>[2x]AVTPPPEKFNFAEHLLQTNRVRPDKTAFVDDISSLSFAQLEAQTRQLAAALRAIGVKREERVLLLMLDGTDWPVAFLGAIYAGIVPVAVNTLLTADDYAYMLEHSRAQAVLVSGALHPVLKAALT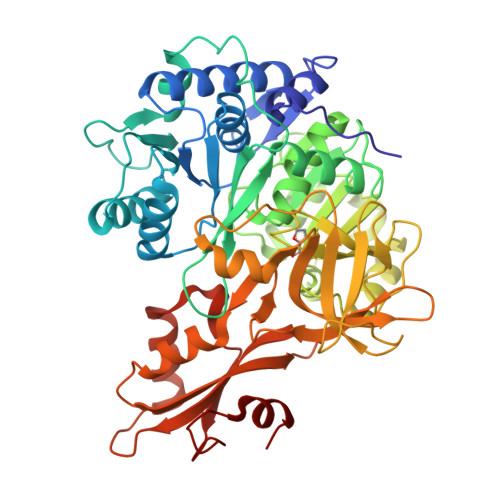KSDHEVQRVIVSRPAAPLEPGEVDFAEFVGAHAPLEKPAATQADDPAFWLYSSGSTGRPKGVVHTHANPYWTSELYGRNTLHLREDDVCFSAAKLFFAYGLGNALTFPMTVGATTLLMGERPTPDAVFKRWLGGVGGVKPTVFYGAPTGYAGMLAAPNLPSRDQVALRLASSAGEALPAEIGQRFQRHFGLDIVDGIGSTEMLHIFLSNLPDRVRYGTTGWPVPGYQIELRGDGGGPVADGEPGDLYIHGPSSATMYWGNRAKSRDTFQGGWTKSGDKYVRNDDGSYTYAGRTDDMLKVSGIYVSPFEIEATLVQHPGVLEAAVVGVADEHGLTKPKAYVVPRPGQTLSETELKTFIKDRLAPYKYPRSTVFVAELPKTATGKIQRFKLREGVLG3-(2-methylpropanamido)benzamide | 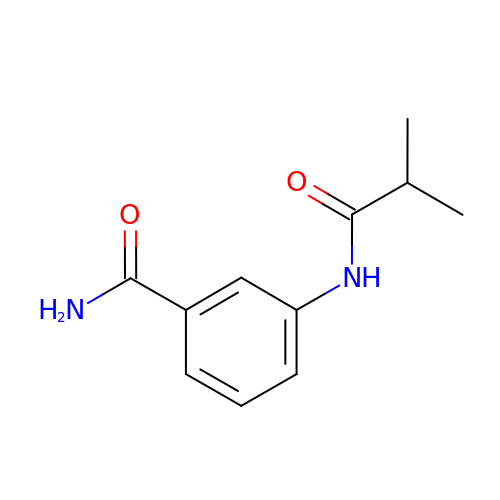C11 H14 N2 O2 | BNDJIHWSAYLUIZ-UHFFFAOYSA-N>[4x]SNAALLTAKTFSLQFNNKRRVNKPYYPRKALLCYQLTPQNGSTPTRGHLINKKEDHAEIR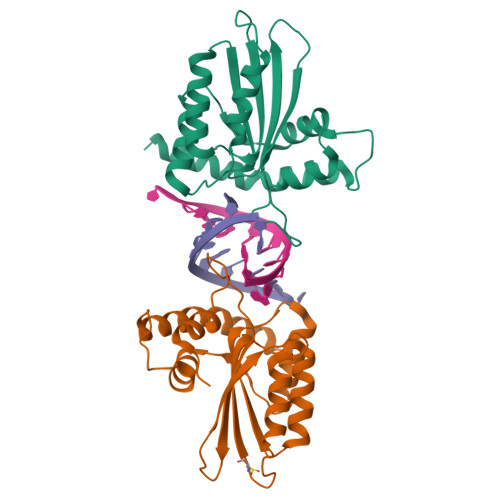FINEIKSMGLDETQCYQVTCYLTWSPCPSCAGELVDFIKAHRHLNLRIFASRLYYHWHPNYQEGLLLLCGSQVPVEVMGLPEFTDCWENFVDHKEPPSFNPSEKLKELDKNSQAIKRRLERIKSRSVDVLENGLRSLQLGPVTPSSSIRNSRGGR> HMAALDSLSLFTSLGLSEQKARETLKNSALSAQLREAATQAQQTLVSTIDKATGILLYGLASRLRDTRRLSFLVSYIASKKIHTEPQLSAALEYVRSHPLDPIDTVDFERECGVGVIVTPEQIEEAVEAAINRHRPQLLVERYHFNMGLLMGEARAVLKWADGKMIKNEVDMQVLHLLGPKLEADLEKKFKVAKARLEETDRRTAKDVVENGETADQTLSLMEQLRGEALKFHKPGENYKTPGYVVTPHTMNLLKQHLEITGGQVRTRFPPEPNGILHIGHAKAINFNFGYAKANNGICFLRFDDTNPEKEEAKFFTAICDMVAWLGYTPYKVTYASDYFDQLYAWAVELIRRGLAYVCHQRGEELKGHNTLPSPWRDRPMEESLLLFEAMRKGKFSEGEATLRMKLVMEDGKMDPVAYRVKYTPHHRTGDKWCIYPTYDYTHCLCDSIEHITHSLCTKEFQARRSSYFWLCNALDVYCPVQWEYGRLNLHYAVVSKRKILQLVATGAVRDWDDPRLFTLTALRRRGFPPEAINNFCARVGVTVAQTTMEPHLLEACVRDVLNDTAPRAMAVLESLRVIITNFPAAKSLDIQVPNFPADETKGFHQVPFAPIVFIERTDFKEEPEPGFKRLAWGQPVGLRHTGYVIELQHVVKGPSGCVESLEVTCRRADAGEKPKAFIHWVSQPLMCEVRLYERLFQHKNPE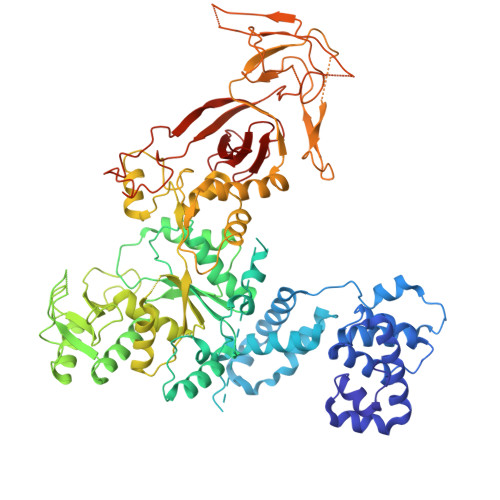DPTEVPGGFLSDLNLASLHVVDAALVDCSVALAKPFDKFQFERLGYFSVDPDSHQGKLVFNRTVTLKEDPGKV> TALPAFNVNPNSVSVSGLASGGYMAAQLGVAYSDVFNVGFGVFAGGPYDCARNQYYTSCMYNGYPSITTPTANMKSWSGNQIASVANLGQRKIYMWTGSSDTTVGPNVMNQLKAQLGNFDNSANVSYVTTTGAVHTFPTDFNGAGDNSCSLSTSPYISNCNYDGAGAALKWIYGSLNARNTGTLSGSVLSFAQSGSYGANGMDTTGYLYVPQSCASGATVCSLHVALHGCLQSYSSIGSRFIQNTGYNKWADTNNMIILYPQAIPDYTIHAIWNGGVLSNPNGCWDW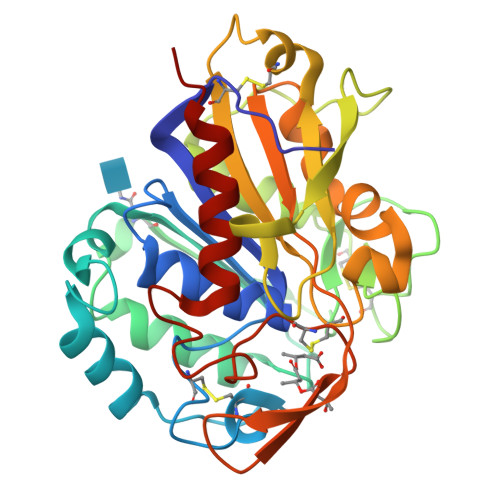VGWYGSNADQIGGVQMAAIVGQVKQIVSGFQ> MVVTFLQDLEVLQDALLNNLQKLSAISRRKESGESKHDNKDSFAAIANEHNDEEEEIEFEDLVNIIESKVSDFESVLKCSIVEMTYKYPELKLQWEKSPRYDQCDKLHIVKLDKQMNEDIYAQLVEELDFVLQFVDWFYCYRLKVKEILRQHHKRDLAWNDEKRDRAIKFHAVDYDKLHQGTSSSSSLTSTSMEKASTREKLLSKTKQLTNNLVRGNQILQSGILQSDLNLDELRAQTNSLTQIDDKYTQFETVFKKTADLVKVLENASHQEKRD;> MAETSNDPFLSYVLSSKQLTNLNRLRRKAVTKQLGSSDDNKVSEEFLRYQHTYQREAFEYLQTKHDAHKIMESQYEQYQSSSKTRRYSIDLDSVDAVDTESQTEYPNEEFIDRNEDSEAVMELRKRLLGKGQNKGLGYETTKSVDRQIEDQDTLQQDLIQDMSKLVGSLKQGAVAFQSALDEDKQVLGAAEIGIQVASQGLMDVSGKLRKYD;> MNGIDDLLNINDRIKQVQNERNELASKLQNLKQSLASNDTEVALSEVIAQDIIEVGASVEGLEQLRAKYGDLQILNKLEKVAVQQTQMQAGVDKLDSFERQLDELAEQPPDQFTLDDVKALHSKLTSVFATVPQINNIDSQYAAYNKLKSKVTGKYNDVIIQRLATNWSNTFDQKLLEAQWDTQKFASTSVGLVKCLRENSTKLYQLSLLYLPLEEETQNGDSERPLSRSNNNQEPVLWNFKSLANNFNVRFTYHFHATSSSSKIETYFQFLNDYLAENLYKCINIFHDDCNGLTKPVIHEQFINYVLQPIRDKVRSTLFQNDLKTLIVLISQILATDKNLLNSFHYHGLGLVSLISDEVWEKWINYEVEMANRQFINITKNPEDFPKSSQNFVKLINKIYDYLEPFYDLDFDLLVRYKLMTCSLIFMNLTSSYLDYILTVDSLNETRTKEQELYQTMAKLQHVNFVYRKIKSLSSNFIFIQLTDIVNSTESKKYNSLFQNVENDYEKAMSTDMQNSIVHRIQKLLKETLRNYFKISTWSTLEMSVDENIGPSSVPSAELVNSINVLRRLINKLDSMDIPLAISLKVKNELLNVIVNYFTESILKLNKFNQNGLNQFLHDFKSLSSILSLPSHATNYKCMSLHELVKILKLKYDPNNQQFLNPEYIKTGNFTSLKEAYSIKYLKDTKIQDALYRIIYGNIL;> MLEEQLYLLACIFASRADTRNIKKLSTRLGSQSKYLEILCVLWPELDDPKNLLFLRELEEEVQSPEGEETTDEDVIVELLESDSSLIPLIESDTTTRSNRYHELQEF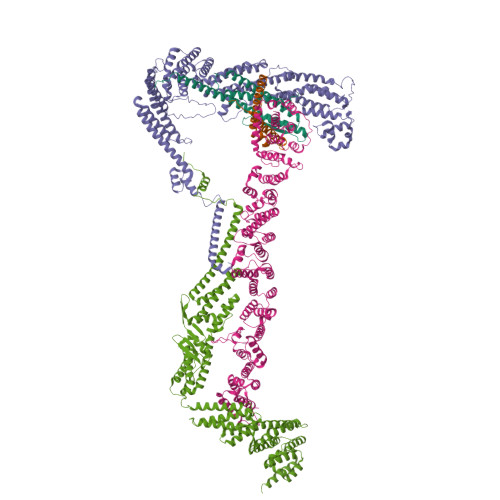ISKKLNNKTLENFEEWLRERILICNEMIPETPLLYSVLWETAKSKVLSTKFIGWVEGVLKPLDHLNKRLHLIFKINEWEKMPDSELFKIIFDGVEDMQGYIGIADVIEDELAPTLSYGKKWETFITEFFNKQQFSLKSDTNYQLFIKLYYSLEKGVKDNSEASRKLQSNVVDILFHNSENLFNLSSLTHKLDELWSILSGFPDEITIEEQKTITALEMKQFMEFFIKCSTKFSFKEIFAITQEEESAQLAHFSSLCHEEFNKANEISSFLQAMYETVLDISKDDKIFTRISMDEKLYSILEILLQMNEFAYIEAIIERFDYSNNTQIYELLVKFFWHFFNNASNGLRKEPEMKKASQTLQIIQKHMSQRAGTNLTKLEVLLEISDKLSHYSINLNKSHNGARDTAFKPSNILEYRDCPLDIISNLLELNPRLYKDLPTTKSLLFGIYDSLSINREGQTGKVEVDLMVLHIDYALVNLDFGTAYELGKQVFEICQEAGQHMMKALGDEHWLTFYQMGKFVDPNWVDNEIPTEIIVLQMSILGRLLEVCPLEEVEIVTSQWSTLELELSARDLVKDKYALDGQNDNKSKVGGIAREIFHNVTNF;> MKHHHHHHHGAAGTSLYKKAGENLYFQGSMESLFPNKGEIIRELLKDPLILKNDSKRSNGSELELDSSDLLQREAILANELNILDNLKTFLNLIKEVKTNLNILELENCYYSLQSLRKKMRNNAAYLKQSFNFQQSISTYVDTLHLELVSTLYKILTNGFWKITENSIQFTPTVEWGKDKVHIEYDTFMDFVAQQYFPKGSLDNQAWFILDMTSADSQEQVRAKLNTIMKEYMNLSRIVSMIKNSIFISGKEISYENEKNILVFSKSSSHGQHCVSTVLTSFEAVCDFMLDGLAFRDRKTLSYELGPLFNTEFTKFVKNNASIILESLDSPLKNLVSVINNKLTRLVAKSEVTNWTHSGKEIQDLLMNKQLYYNLLLDKVLESHISEIRSIFEDPKKSWQNLEVVELTTSNTNTMSEKIGKNDSDVQNEKELHNAVSKDDDWNWEVEDDDADAWGDEIDVNIDDEEEKTNQEKEKEPEEEENAWDEAWAIDENIDDASLENGKEHLKAHDVGSLDKDHIEVTQLPKLFLAISQNFKSSFADSHVDEQYFAYKYNLLQTSYMAMCTANFSHNWCQLYVDMRYLIERDEKLYRIKELTRNLLETKLNMKYRIVCQLIRHQLTEFRENERNPSWDATIEKLLPYILKEIVRPLQKIRGEEGSRYLLSFLNFLYNDCVTKEILKWQIISEVNSENLGELVSLLVNNTDIQLLAKEPSYKKMREKFATMGKFLPLHLKEIMEMFYNGDFYLFATDELIQWIELLFADTPLRRNAIDDIYEIRGTALDD>[4x]MAQHTVYFPDAFLTQMREAMPSTLSFDDFLAACQRPLRRSIRVNTLKISVADFLQLTAPYGWTLTPIPWCEEGFWIERDNEDALPLGSTAEHLSGLFYIQEASSMLPVAALFADGNAPQRVMDVAAAPGSKTTQISARMNNEGAILANEFSASRVKVLHANISRCGISNVALTHFDGRVFGAAVPEMFDAILLDAPCSGEGVVRKDPDALKNWSPESNQEIAATQRELIDSAF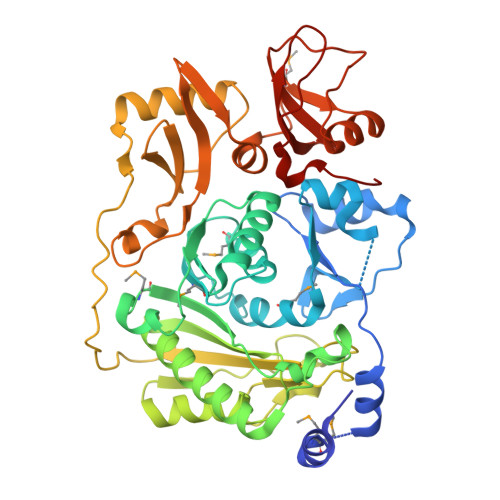HALRPGGTLVYSTCTLNQEENEAVCLWLKETYPDAVEFLPLGDLFPGANKALTEEGFLHVFPQIYDCEGFFVARLRKTQAIPALPAPKYKVGNFPFSPVKDREAGQIRQAATGVGLNWDENLRLWQRDKELWLFPVGIEALIGKVRFSRLGIKLAETHNKGYRWQHEAVIALASPDNMNAFELTPQEAEEWYRGRDVYPQAAPVADDVLVTFQHQPIGLAKRIGSRLKNSYPRELVRDGKLFTGNA> GPGSASPDLLSEVSEMKQDLIKMTAILTTDVSDKAGSIKVKELVKAAEEEPGEP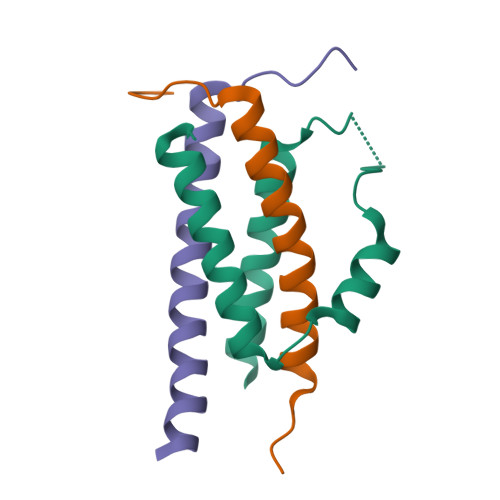FEIVERVKEDLEKVNEILRSGT;>GPGSGFGTSPLTPSARISALNIVGDLLRKVGALESKLAACRNFAKDQASRK[2x]>[8x]MDVGKLESFIVEKMAERKVPGISISIIKDGDVVYAKGFGYRNVEARLPSTPETIYGIGSITKSFTALAIMKLVEEGGLSLDDPVEKFVNIKLRPFGEPVTVHHLLTHSSGIPSLGYAEAFIDGMVGGDNWLPVSTPEETIAFARDMEKWAVAKPGERFFYLNTGYVLLGKIIEKVSGVSYEEYIKKKILEPLGMNRSYFFKEEVEKDKDVAMGYILDKEGRLVPQPFPYGITADGGLLSSVLDLAKYLKMYIERDESIVSKEYIEKMETSYIKVPWEIFGGEGYGYGLIIYPNFLGEKLVGHSGSVGMYTGYIGYIPEKKIGVAVLENSSGYPPSYIAMYALALLLGKNPEKELPFIYRERILKKVEGRYMGYKGTIKFEVKVDGDVVYLRALGRAFTYTIPLFPEVLEEDFIKCYTLSNGRKMYAEFYIKDNKVDLIFERYRLIKS

Pab87 is a serine protease belonging to the MEROPS S12 family and displays sequence similarity with penicillin-recognizing proteins, termed PRP. Pab87 is the first characterized member of a new self-compartmentalizing protease family, referred to as CubicO proteases as they display a cubic-shaped octameric form. In conclusion, Pab87 is a hyperthermophilic peptidase that acts on d-amino acid containing peptides at N- and C-termini. Taken all together, we propose that CubicO proteases play a central role in proteolysis of these bacterial cell debris that contains d-amino acids.

The Pab87 structure was determined at 2.2 Å resolution using the single-wavelength anomalous dispersion method with anomalous signal of a high-phasing-power lanthanide derivative, the Lu-HPDO3A complex. The crystal structure of the P. abyssi CubicO protease (Pab87) reveals a 422 symmetry, where the eight monomers are arranged in a barrel-shaped architecture. In the protease complex, monomers associate through a non-crystallographic four-fold axis to form two stacked tetramers that are themselves related by a non-crystallographic two-fold axis perpendicular to the latter. The 50.4 kDa monomer of Pab87 consists of two structural domains, an N-terminal PRP domain associated to a C-terminal lipocalin domain that plays a crucial role in the octamerization and in the active site compartmentalization. The N-terminal domain structure follows the pattern of the known PRP structures, composed of two regions, one α/β and one all-helical region with six helices. The Pab87 C-terminal domain presents a typical lipocalin superfold that consists of an α-helix and an eight-stranded antiparallel β-barrel. Each monomer interacts with four other subunits of the octamer but main interactions are observed within the head-to-tail dimers, where monomers interact primarily with each other by shape recognition through key-lock type interaction. Intersubunit contacts are formed by electrostatic and hydrogen-bonding interactions between the bottom of the lipocalin domain of the first monomer and the all-helical region of the PRP domain of the second monomer. The 20 Å wide square-shaped channel, running along the four-fold axis through the entire complex, joins the equatorial two-fold axes into a 60 Å wide central cavern formed by association of the eight C-terminal domains. Each active site, facing the central cavern, lies between three domains, the PRP and the lipocalin domains of one monomer, and the second lipocalin domain of a head-to-tail dimer.Nonsense-mediated mRNA decay (NMD) is a eukaryotic mRNA quality control mechanism that recognizes transcripts with premature termination codons (PTC) and promotes their degradation. Human UPF2 (Q9HAU5) is an ∼140 kDa protein containing three conserved MIF4G (Middle portion of eIF4G) domains that are found in a number of proteins involved in RNA metabolism and translation such as the nuclear cap-binding protein CBP80 and eIF4G (eukaryotic initiation factor 4-gamma). UPF2 interacts via its third MIF4G domain with UPF3b and via its C-terminal extremity with UPF1, thus forming the central component of the ternary complex of UPF proteins. Here, we present the atomic resolution crystal structures of the N-terminal (MIF4G-1) and middle (MIF4G-2) domains of UPF2 and a lower resolution crystal structure of the combined UPF2 MIF4G-2/MIF4G-3 domains.

The crystal structure of UPF2 MIF4G-2 (residues 455–757) shows that the core MIF4G fold of 10 antiparallel helices (residues 561–756) is preceded by an ∼100 amino acid region (residues 458–560) that contains additional elements essential for stability. The first part of this N-terminal region (458–478) folds into two short α-helices (hA and hB), which together with the connecting loops pack against helices h2, h4, h6 and h8. The interaction is mainly hydrophobic, involving Ile458, Trp459, Phe467 and Tyr468 of helix hA and Pro620, Phe621, Phe676 and Phe713 of h4, h6 and h8. Two salt bridges are also established between Glu460 and Arg712 and Arg716 on helix h8. Helix hB and its adjacent loops pack against helices h2 and h4 via hydrophobic interactions. Residues 481–558 following helix hB are largely disordered in the crystal structure (apart from the short helix hC) and indeed this region is highly variable between species. Similar to MIF4G-1, the N-terminal region stabilizes the interhelical packing of the MIF4G-2 domain helices. In fact, residues 458–478 are evolutionarily conserved within UPF2, and the expression of MIF4G-2/3 constructs lacking this capping region yields mostly insoluble protein. Notably, superposition of MIF4G-1 and MIF4G-2 shows that the capping helices hA and hB in the two domains pack against the same region of helices h2, h4, h6 and h8. We solved the structure of UPF2 MIF4G-1 and MIF4G-2 domains at 2.6 and 2.4 Å resolution, respectively, using SAD on seleno-methionine substituted protein crystals.

> GAMGEGGIWEDEDARNFYENLIDLKAFVPAILFKDNEKSCQNKESNKDDTKEAKESKENKEVSSPDDLELELENLEINDDTLELEGGDEAEDLTKKLLDEQEQEDEEASTGSHLKLIVDAFLQQLPNCVNRDLIDKAAMDFCMNMNTKANRKKLVRALFIVPRQRLDLLPFYARLVATLHPCMSDVAEDLCSMLRGDFRFHVRKKDQINIETKNKTVRFIGELTKFKMFTKNDTLHCLKMLLSDFSHHHIEMACTLLETCGRFLFRSPESHLRTSVLLEQMMRKKQAMHLDARYVTMVENAYYYCNP>MEIRGLLMGRLRLGRRMVPLGLLGVTALLLILPPFALVQGRHHELNNGAAIGSHQLSAAAGVGLASQSAQSGSLASGVMSSVPAAGASSSSSSSLLSSSAEDDVARITLSKDADAFFTPYIGHGESVRIIDAELGTLEHVHSGATPRRRGLTRRESNSDANDNDPLVVNTDKGRIRGITVDAPSGKKVDVWLGIPYAQPPVGPL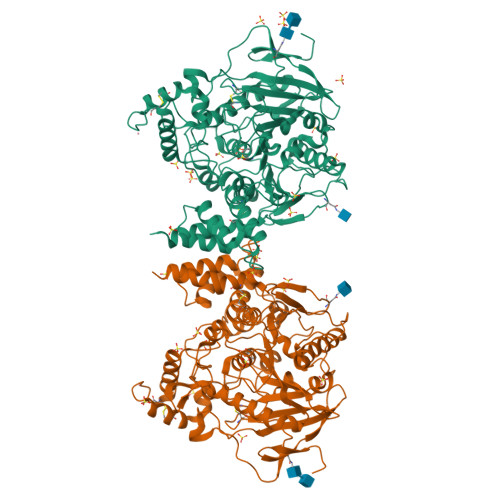RFRHPRPAEKWTGVLNTTTPPNSCVQIVDTVFGDFPGATMWNPNTPLSEDCLYINVVAPRPRPKNAAVMLWIFGGGFYSGTATLDVYDHRALASEENVIVVSLQYRVASLGFLFLGTPEAPGNAGLFDQNLALRWVRDNIHRFGGDPSRVTLFGESAGAVSVSLHLLSALSRDLFQRAILQSGSPTAPWALVSREEATLRALRLAEAVGCPHEPSKLSDAVECLRGKDPHVLVNNEWGTLGICEFPFVPVVDGAFLDETPQRSLASGRFKKTEILTGSNTEEGYYFIIYYLTELLRKEEGVTVTREEFLQAVRELNPYVNGAARQAIVFEYTDWTEPDNPNSNRDALDKMVGDYHFTCNVNEFAQRYAEEGNNVYMYLYTHRSKGNPWPRWTGVMHGDEINYVFGEPLNPTLGYTEDEKDFSRKIMRYWSNFAKTGNPNPNTASSEFPEWPKHTAHGRHYLELGLNTSFVGRGPRLRQCAFWKKYLPQLVAATSNLPGPAPPSEPCESSAFFYRPDLIVLLVSLLTATVRFIQ[2x]>[6x]GQPASPPVVDTAQGRVLGKYVSLEGLAQPVAVFLGVPFAKPPLGSLRFAPPQPAEPWSFVKNTTSYPPMCCQDPVAGQMTSDLFTNRKERLIPEFSEDCLYLNIYTPADLTKRGRLPVMVWIHGGGLVVGGASTYDGLALAAHENVVVVAIQYRLGIWGFFSTGDEHSRGNWGHLDQVAALHWVQENIANFGGDPGSVTIFGESAGGESVSVLVLSPLAKNLFHRAISESGVAFTAGLVRKDMKAAAKQIAVLAGCKTTTSAVFVHCLRQKSEDELLDLTLKMKFFALDLHGDPRE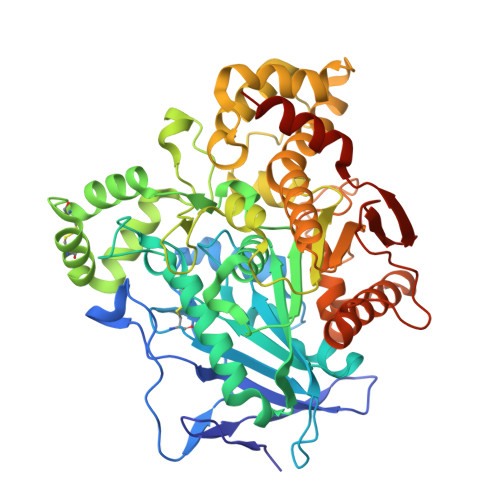SHPFLTTVVDGVLLPKMPEEILAEKDFNTVPYIVGINKQEFGWLLPTMMGFPLSEGKLDQKTATSLLWKSYPIANIPEELTPVATDKYLGGTDDPVKKKDLFLDLMGDVVFGVPSVTVARQHRDAGAPTYMYEFQYRPSFSSDKKPKTVIGDHGDEIFSVFGAPFLRGDAPEEEVSLSKTVMKFWANFARSGNPNGEGLPHWPMYDQEEGYLQIGVNTQAAKRLKGEEVAFWNDLLSKEAAKKPPKIK>MSKSPYVDPHKSGHEIWEEFSMSFTPAVKEVVEFAKRIPGFRDLSQHDQVNLLKAGTFEVLMVRFASLFDAKERTVTFLGSKKYSVDDLHSMGAGDLLNSMFEFSEKLNALQLSDEEMSLFTAVVLVSADRSGIENVNSVEALQETLIRALRTLIMKNHPNEASIFTKLLLKLPDLRSL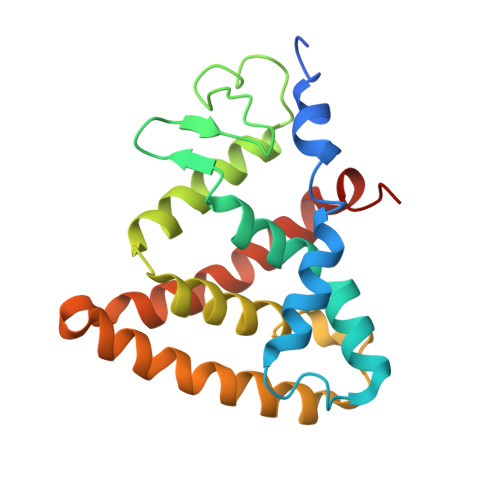NNMHSEELLAFKVHP[4x]>[4x]KL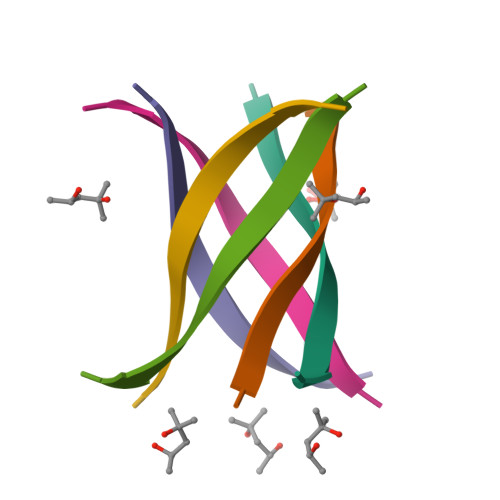KVLGDVIEV>TKPLDGINVLDFTHVQAGPACTQMMGFLGANVIKIERRGSGDMTRGWLQDKPNVDSLYFTMFNCNKRSIELDMKTPEGKELLEQMIKKADVMVENFGPGALDRMGFTWEYIQELNPRVILASVKGYAEGHANEHLKVYENVAQCSGGAAATTGFWDGPPTVSGAALGESNSGMHLMIGILAALEIRHKTGRGQKVAVAMQDAVLNLVRIKLRDQQRLERTGILAEYPQAQPNFAFDRDGNPLSFDNITSVPRGGNAGGGGQPGWMLKCKGWETDADSYVYFTIAANMWPQICDMIDKPEWKDDPAYNTFEGRVDKLMDIFSFIETKFADKDKFEVTEWAAQ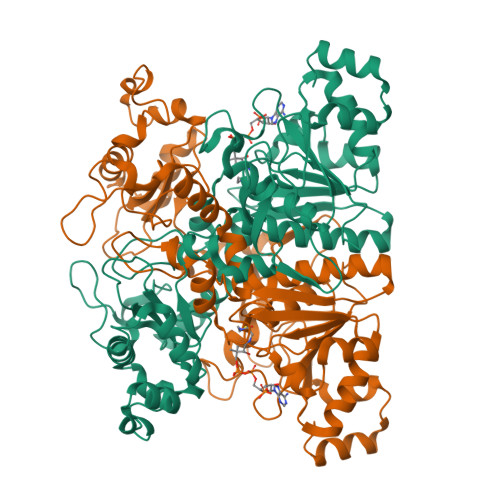YGIPCGPVMSMKELAHDPSLQKVGTVVEVVDEIRGNHLTVGAPFKFSGFQPEITRAPLLGEHTDEVLKELGLDDAKIKELHAKQVV[2x]The structure of PolI_G20c was solved with the aid of the structure of an exonuclease termed ExnV1, which was determined in parallel in this work and originates from an Icelandic virus metagenome collected from several hot springs in Iceland. The gene coding for ExnV1 may be part of a truncated gene that originally encoded a DNA polymerase I. A novel structural motif, SβαR, that was not previously associated with DNA polymerases I was identified in the solved structures of ExnV1 and PolI_G20c. Residues 152–185 are missing in chain B of PolI_G20c; however, the residues corresponding to those in ExnV1 are present and from the sequence alignment it is interpreted that PolI_G20c also resembles ExnV1 in this area, which is part of a novel structure motif (SβαR) that is discussed further below. The major difference between the two proteins is that ExnV1 only comprises the smaller 3′–5′ exonuclease, whereas PolI_G20c also includes the larger palm domain that is responsible for the polymerase activity. The SβαR structural motif consists of two β-strands followed by two α-helices that are connected to each other via a short β-strand.

Sequence and structural analysis of PolI_G20c revealed a 3′–5′ exonuclease domain and a DNA polymerase domain, and activity screening confirmed that both domains were functional. Since ExnV1 only includes a 3′–5′ exonuclease domain, the gene encoding ExnV1 is most likely to be truncated. It is concluded that PolI_G20c belongs to the DNA polymerase I family but lacks the typical 5′–3′ exonuclease domain. With these data at hand, the structure of PolI_G20c was determined to 2.97 Å resolution. The structure of PolI_G20c consists of two polypeptide chains, A and B, that could possibly be arranged as a dimer according to PISA structure analysis in CCP4mg. In PolI_G20c the supposed two long β-strands are only seen as one-residue β-strands 8 and 9, since there is a gap in the structure, although if all of the amino acids in the structure were seen we propose that they would resemble the long corresponding β-strands in ExnV1. The maximum activity of PolI_G20c and GoTaq was measured at about 70°C, while IsoPol BST+ exhibits maximum activity at 65°C. IsoPol BST+ also exhibited significant activity at temperatures below 40°C, whereas PolI_G20c displayed very limited activity below this temperature.

>MRSYHVVTNDTLPSALDAIAQAPRVALDTETYGSNPFNLYLPDFRLVGVAIATSPTEAWYFPVDHQDFLLRYQPANLPREAVRQAVLEALKRPVVYHNAAYDRRVLAVTLDIPLDQTYGDDTMVALHLVDENHPLGLKEWAKTLLGLEEVNADIEPPELTDEDQVEAVSKNGRRYKKKVHKLKPDWLQRLKDAFLAVHNGGVSYSALYKLLNRAFQQLKNRGVVSYTGSFPNDFRLFPVDIAAIYALDDAMNTLALWEHVEVFFELHPKLHALYREIELPVNDVMTRATHRGVLVDKEELRRIKETIQARIEEKAQEAQELLKALIGSKASEFTNPLNSPQQLSTILYDLLGYPVVETTPNGAPSTSKTAIAKLLTLSPKDKRKAPLAKAFLEAKQAHEGLKKLLSTYTDSILEEVDPQGRLHTNFNTVGTVSGRMSSSNPNLQNLPRLLPEEVAEKPYLQGIDIRKAFVADPGYTFVSADYASMELVVCAAVSGDPTMRDLLNQGRDLHAYTARYAFKVGLDLDDKAFKEQYKDYRQKAKVVNFALIYGGTEFTLIKNFGFSEEEAKQLIQGYFEAYPVVKTWMEEVYRELEEKGFVEYPIYGYIKRMDLPQALRKLPKDKWPLVLNNDPDARKQYYASLRSCQNALIQGFSAFVVKDAIVQMQRAFEAEGLDAQVIIQVHDEIVVLAKEEHAERVAQIMVEKMEREVNGVLLKAEPEFKRTLSKVGLEHHHHHH[2x]>[2x]PISKMVTAHFVLIHTICHGAWIWHKLKPALERAGHKVTALDMAASGIDPRQIEQINSFDEYSEPLLTFLEKLPQGEKVIIVGEACAGLNIAIAADRYVDKIAAGVFHNSLLPDTVHSPSYTVEKLLESFPDWRDTEYFTFTNITGETITTMKLGFVLLRENLFTKCTDGEYELAKMVMRKGSLFQNVLAQRPKFTE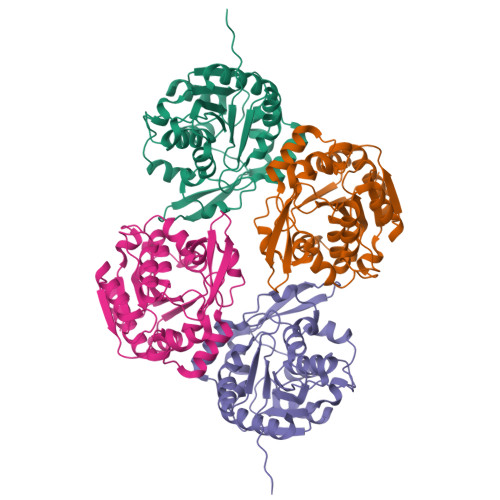KGYGSIKKVYIWTDQDKIFLPDFQRWQIANYKPDKVYQVQGGDHKLQLTKTEEVAHILQEVADAYA> MAAQLALNSEASLWGPYREIWQTVLSALIKRQPEAVHSLDIVLKKYKPDFISLFKNPPKSAQQHERVQKASTEGIPIKGTQRTRILEEQLIKEAFILSDLYNIGEIAAVELLLIGEQQQPTFHGLTRGLVAILLYWDGKSCMAESLLHLIQARKGKTFTLDHSPEVVSMVTRFTDDLMEQGLTNKILTLISQIDVNNEFDKLKKERGLGNKKHRKEVSDLIKECQQSLAHSLYSWSCQTPLNREDTLLLIGYLEKVTVEGDGSLDKVNLTLLMSLLYCLDVGFLEQGTDDREELMKQASMFMDRQYIAAIHNRLQNTQPWKSPGMQATVRLAWALALRGISQFSEVLEFSEADEPMAEIAIGGNVFLFLTEAVVGSESFCTDEFFIRRIHKLVTDFPTLMPMKVKQLRNRAEEDARLIQMSMQMGNEPPASLRRDLEHLLLLIGELYRKDPFHLELALEYWCPTEPLQSTSLMGSFLGVAHQRPPQRQVLLSKFVRQMSDLLPATLYLPYLKMLRGLASGPQCAHYCFSLLKANGGSSAENLQAAGGSPVSWDHFFHSLMLYHEHLRRDLPNTDNIHQRHPPLRGITQRELDGLIACLQLTCTIIDWSESARLALCEHAQWMPVVVILGLLQCSIPPLLKAELLKTLAAFGKSPEIAASLWQSLEYTQILQTVRATGLRQGVGIEVELNEIESRCEEYPLTRAFCQLISTLVESSFPTNLGAGLRAPGFEPYLQFLRDTVFLRYRTRAYRRAAEKWEVAEAVLDVFYKLLKDYEPQPEDFVDQYVELQGEERVAFKPPGFSLMHHLLNESPMLELCLSLMEEGVTQLDTYAPFPGKKHLEKAVAYCFMLLNLTLQKENRFMDLLRESHLSMIVTPLEQLLQGINPRSKKADNVVNIARYLCHGNSNAELAFESAKILCSISCNSKIQEKIVGDFTQDQNVSQKLMVGFVSCLDSEEAEELLDSEKEAEDQVKQTNIRYMTKIHILNLLITSLEMKAPNLAMFLLGYELKKPVSTTNLQDSGVLGCPRTCLHSILDILRKGTDVRAGPVAVWDTPHLAELCYQVIYQLCACADTSGPTMRYLRTSQDFLFSQLQHLPFSVEESEISAMNQMSWLMKTATIELRITSLNRQRSHTQRLLHLLLDDMPTRPYSADGEGGMEDESRSLSGFLHFDTTSKVRRKILRILDSIQFSNEIPEPLQLDFFDRSQIEQVIANCEHKNRRGQTVCNVKLLHRVLVAEVNALQGMAAIGQRPLLMEEINTILQYVVERNKLLQCLHAKRHALESWRQLVEIILTACPQDLIPTEHRQLIIRDLLQDLHVKILDDDAAQELMPIVAGAVFTLTAHLSQSVRTELKQPMTASGLGQSQYVQMLDGSFAAPPGTENISAGFASIGDSSLHMILRNLLEFILKTGGGFQRVRAHLYGSLLYYLQIAQRPDEPDTLESAHKSMWERLTAPEDVFSKLQRDNLSIFESYGTALMEVVCRDACDGHDIGRMLALALLDRIVSVDRQQQWLLYLSNSGYLKVLVDSLAEDDVVLRNLLTPQPPLLKALYIYESKMAFLTRVAKSSQGAIELLRSGVIVRLAQCQVYDMRPETDPHGVFGMRETPVFIPAPVERYRQILLPALQICQLILTSSTAQHLQAAGQVLQFLVAHSDTIQAILRSQEGSLGSLQELALLTGIISKAALPGVLNELDIGLNDGSMMELQGHIGRFQRQCLALLNRFGGSDRLRQLSLQDDSSRLDGVSKKDDMELAMQQICSNVMEYCQALMIQNSPSFQQTVCLFTPSLKESASRDGTRQDSQVSILPSWRLPSLGVVIHLLKQSANNFFTYYDIHRQSVGKLQNVEQLPPDEIKELCQSEMPVGADKISTTQKYGLARRRLVKLINSRAKLLSLCSYIIETCLYILWRHLEYYLLHCTTSDSQDPVFSNMTFGNRRFQDTFNTDPNMDPRNLRQNKVSQQDVDTLLREGANSFGESLQKRLLDIESLYCKVRSRHSFIQALVRRIRGLLRVSRV;>MEELDVDPAETPIPGLGQQNRHIGFSWGPGDLLLYETLYQKQGNSETAARCPFMYLVRSDEDIYSPVLRKLFNESHSIFVGLQKSAEEASGKSRKAQLVQVSRNYRSVLRACMEEMHTLSESTRETAQKYISQISILSAMELSWNLCEILFIESAPAGPLLILLLEWVRLHVCEVDNIVQDVLRSEKPTEHEKFWDGVTGYVLQGRMNEARQLLAKEASTSASARSMCRVLDDLLKKMPMLHTGGTQTLTEFELKWQHWREECERHLQNGTFSSNVHMEAVCRVLLGDEEVLLEKRDLMTTWYHFLVSRLLFKHPTVKPTELHFYAQSSLDMFLAGDSCPEPLDNILLAAFEFDIHQVIKEFSIVSSNWWFVAHLTDLLDHCQLFQAHNLYFGANMREFLLLDYASGLFSHHSLWQLGVDYFDYCPNLGREYLKLHMERIPLSTEKKALKALRICEQRQMTEQVRSICKTMAMQSLCNRRLGSALSWSIRAKDAAFATLISDRFLKEYCERGNFTDLDLIDNLGSAMLLSDRLTFLGKYREFHRMYSQEQFSEAASLLLSLMTARIAPCSFWLTLLLDALPLLEQKQVIFSAEQTYELMRCLEDRMAAKLESTSPDEIQKQDSSIDNTKVEMLRLALARNLARAIVTEGALQE[2x];>MADKFAAKFVSHKISRTRWRPVSASSLQQPDVFATGSWDNEENKVCVWATSDFGATSLDEEYQGDPKQLCDIKHPGDVMDMQFLDKERIVTGSSTGTVTIFRHHENNQTLSVNQRWEQAHYHVGSNMRAPCTAIVCSSPEIVSVGEDGRINCFRAESRDVLRTIDDADSSTMHGVTFLRTTEILTVNSVGQLKLWDLRKQGNDPTQIFSVTGERVPLHCVDRHPNQQHVVATGGQDGMLCIWDVRHGKMPMSLLNAHEAEMWEVHFHPSNPDHLFTCSEDGSLWHWDASADSEKPTFLLGGRSTFNISRSSIAPPNANQSLACAWLSTDPTKGQLEITNLLPSSTLSVNSLDVLGQNLVCGTDAEAIYVTRRLFS[2x];>[2x]MFVARSIAADHKDLIHDVSFDFHGRRMATCSSDQSVKVWDKSENVNWHCTASWKTHSGSVWRVTWAHPEFGQVLASCSFDRTAAVWEEIVGESNDKLRGQSHWVKRTTLVDSRTSVTDVKFAPKHMGLMLATCSADGVVRIYEAPDVMNLSQWSLQHEISCKLSCSCISWNPSSSRAHSPMIAVGSDDSSPNIMGKVQIYEYNENTRKYAKAETLMSVSDPVHDIAFAPNLGRSFHILAVATKDVRIFTMKPLRKELSSSGGVTKFENHTVAQFDNHNSQVWRVSWNITGTVLASSGDDGTVRLWKANYMDNWKCIGVLKGDGNPVGNSFQGIFGSSIGSASHGLQNSVNGTSTSGRKHS;>MAAAERHMTPFQAIDWAGSITLPMVQRVGGFTRAIMAASVNLERSYMELIGAERETSRRNFRDLSLRPDVNLVIGGPKYADCAGGYCYSESSSLLSATRNRFLHWTSYADTLELVEISLDINLVNNAVRLRILNCSILPGGVHICETPNNIVVLILTNQTVHRLILPHPSRMYRSEIISDSHIQSIFTDIGKTNFHDPSNTYVIPAIPGRAPNTTASTAWLSSDGEALFALPSISGGILVIKMPPHDMEGLVTIAELKQSSVMQRLLTGWMPSSIRGDQGPAHLPVSLAVHTLDHDSYLFALCQDHKLRMWSYKDQMCLMVADMLEYVPVSKDIRQTAGTGHKLRLAFSETLGILYLGVYLHTPKQGQFCVFQLMCAESNRYSLDHISSIFTNQETLIDFTFTLTSMDIWALWLDDDNQTVVKHINFEENQAGQWNPVFVNPLPEDDLAISDEQEPQEAYLECLFAPGRFTIAAVQKAIQILRKGSGRVLDLSWEELRKDVTLTVENEIQNAVIDYDVSQEEFRQINIENWCKFYTCCLQYQETLSRPLALLVHPDTNMVCLLRKGFLSFLAPCSLVEHLYLVPAEHLLTVDESVISDDIDAASDIVNLIQCLRMIADYISEDMAYLMESACCHLQSPERVAEQILEDLIANDIDNIMENIQNKLQDTRNPIRAIGFLLQNMDYETNADMEQPQPNTRLNLSTLYGSITASSVVCQAICKISATRFLICRDLLILQHLLLRLGDMALIGAGQLLHSQQELIPRAAQLLLSYYMIRWGSQCLACAVPVDILESNLQHLSVLELSDSQVEKRRYTSGIQTIVELFFEDVARKHFPHVFIQSGASQLQEPLNWSDLIKRITNYLLQLLWPSNPNFQFAECLMRNCQYTQLQEYVRLLLPWCQVNVGSCHFMLAQCYLVAGEGHKALDCFSQAASEVEREDFLEKLIRVEEGESVSPRLQYYNRVLRLLEDVGLPELVIQLATIAIGEASDDWRSQAALRTRIFKHHLDMGHNNQAYDALTQIPDPSRQLDCLRQLVVVLCERSQLQDLVEFPYVNLHNEVVGIIESRARAVDLMTHNYYELLYAFHIYRHNYRKAGSVMFEYGMRLGREVRTLRGLQKQVNSYLACLNCLRLIRPEYAWIVQPVSGAVYERPGASPKRNYDGESSAVPSSSQIEILELRDLEKEYVLAQTRLTLAKHNPSTAAIAGSSAAEEMVALLVQAGLFDTAISLCQTFKLALTSVFEGLACKCIRLQQGGEAAQAEAWEWLAANQLATVITTKESSATDEAWRLMISYLDKYEAKNTLYHHCIINKLLSHGVPLPNWLINRYKAMDAAELLRLYLKYDLLEEAAELVLEYVDALLGKGHQYFGIQAPLSATSQLVWFPYSAIDHLRQALGENESNQHNQAILSKLQRKMDEYFQKLKKATDDYKKLVQKPLRA[2x];>[2x]MKQDSASNATYTVDCEDYVHVVEFNPFDSGEAGSLLAYGGISYVVIASCRFQEEDSTVEGIEFKTLKTFHHGERVVAIAWSPETRCDALLPLLRFATAAGDKKIRIFTSDFQDKNEYKVIEGHSGYINDLVFCSPEGTDIASVGDDHTCRIWDLDGKQIAMFILRSPGMSVAWHPEGAFKLMVAEKTGTIRFYDLTTHQAILSLESVQVPLMSADWCVRNTLRIGAVAGNDWIIWEMPRSSYPQDNKPAHADRARMFRWSKCNENVFATTGYPGKMKSQIAIHHLAHPQPILIGTAPVGSGLSWHRRLPLCVVGGYRKLFFWLTEM;>[2x]SKYGLQDSDEEDDQLNNAEAKKLKAAPVPPQGKPPPLQQATLPGKVTPPPQSPAVDQLDRVLELDSDMADITQDQDLDSVAEEQDITEEQEPLSASSHIASSLGINPHALQVMKASLLLEEEDGEMINRFSSFPSSMDPYPDVRSPRLFPSSHAKRTSSMGLLQSKFASPSISRISETAQGSHSPRILPVTPWSVPAPLAPTFVIPRPAPETHLRTVGTRRQQELVPLEKSVTHGRGSLLIDMGLFMGRSFRVGWGPNWTLVHNGDKLTERLNAEEDQNMDTIDYGFLPKPTSAKSLTESPFKVHMEKLSLEQKSRELQSYLMPLEIELKNSSVDRSAQCPHFKPNAGVAAIHDYAGWVRNLSNEAGELEAVVKQWGLTWTLCESLWGQLKELEASLDEPNEYVRNLERRKAFSHWLAHTAEERIEEEVSLYGPERHVEAVFSFLTGGRISDACRLAQKSGDHRLSLLLSQMVGSQEMRELISLQLVDWNKLQVDHYIQEERLRVFCLLSGTPVWRSSDNRSINVCSQLDWKRTLAVHLWYMLPPTATIAQALRLYERAFQEHEEGEPYACYPLPPYLEDCSISLGDEPSAKFSSLQRDVCVHLLKLYSERQYDLCQLLDPSSVTPDPLDYRLSWHLWMVLQALNYTHLSEHRQGTLHASYAAQLENVGLWEWAIFVLLHIPHPHIREAGVRELLNRQCVVRESPESLAKENFLIHRLCVPAQWVHEAKAIRSRRDGDRHKEALYLLKGHQWNPCHKLVTRHLAADAVINENYRYLQSFLGELSNPEHCKHIQDWETAGKVYLDYIRVIDMLNLIQQDESSGCELEKLHTKVMSLCKWVELIHCYTAKDRLAQSEMAKRVANILRVVLSLQQPPESMSDSSEPRVPLRLLAPHIGRLPMPEDYALEELRGLTQSYLRELICDS;>[2x]MVSVINTVDTSHEDMIHDAQMDYYGIRLATCSSDRSVKIFDVKNGGQILIADLRGHDGPVWQVAWAHPMYGNILASCSYDRKVIIWKEENGTWEKTYEYTGHDSSVNSVCWAPHDFGLVLACGSSDGAISILTFTGDGPWEVKKISNAHTIGCNAVSWAPSVIPGSLVDQPSSQKPNYIKRFVSGGCDNLVKIWREEDGQWKEDQKLEAHSDWVRDVAWAPSIGLPTSTIASCSQDGRVYIWTSDDAATNCWTPKLLHKFNDVVWHVSWSITANILAVSGGDNKVTLWKESVDGQWACISDVNKGQGAVSTVTEGQLNDQ;>MDMLSPVVREAEVSRAARRQSSNRKNPADESWSNATPTRGPSSRTTGQTLFRQHMTPQTWNSSRPPDVSAILGTVGRSPRLLQTPGRLANLSMMSNPDDSVWTTTFSPGRTGMYTTLDSPSFTEDITLSAVMLQEEDPGEAATMSMYPDFLKSFLEHPSSAVFELIEQYEATCNTQITLLKKIVKRVTPGQQKFSKTASILWLLQQEMVTWRLIAALYRDRIQSALEEENMFEIAAPNASEKTIVDKLFQRDTLVRQSQLVVDWLESIAKDEVGDFSDNIEYYAKSVYWENTLHTLKQRSMLSLGSSRPLVSELDPDAPIRQKLPLDDLDREDDIRLLKYLFTLIRAGMTDEAQRLCKRCGQAWRAATLEGWKLYHDANINGGTELQAVEGNPYRCVWKTCCWRMAEDEQFNKYERAIYATLSGNLKQLLPVCESWEDTVWAHFKVMVDSLVEQEIRASIISFNEANELPREYLEANWTLDSVFEELQATDKKRVLEENREHYHIIQKFVILADVDGLMDEFSEWLSNGKNLLLGHLLRFMTHLLLFFRTLGLQAKEEVSVEVLKTYIQRLINEKQIELIAFYVSHLPQELAISQYAVFLENITDPDQRQRCLELAKEAGLDVASITKTVVENTRKKDAGEFAHHDFAPALDSGTSEEDRAKIDVIDWLVFDPAQRAEALKQSNAIMRKFLASKKHEAAKEVFAKIPQDSIAEIYSQWEEQAMDSALPAEDDNAIREHLCIRAYLESHEAFNEWFKHINSPPQKPTLVGQASFTEKVAHEHKEKKYEMDFGIWKGHLDALTSDVKEKIYNVLLFVDGGWMVDVREDTEEDPERSHQMVLLRRLCLPMMCFLLHTVLHNTKQYKDCLRLADIVSSENQKLYTVFSKTEMRNLLQKLRESSLMLLDLQLDPLGYEIQS[3x];>MFPSPRAQGMGSARRPFNSRLTGGRKALGPGVTASSSPSALYSPVGRRVSASGARSTPSRVYLHPAASETVNYNVQLFGSSLPVKVMEALSNASADEPMAACIHEGGWAWLACNDRLIIWKISHSSSAKLMVCKELPLPLSDSEWSADLVDICAQTGDPAAAQSVALMAATPEGSSRYWPNILHEGTYIESYTEFGSSLCAFVTAVKGNSFILSSEKNQLVRLTPDASGKMNQRVLPQGQGMLSGIGRRVSTLFGILSPAVESTLCSVLWDKGDCFYTLTDSSINKWDLDDTSESQVLNWDMSRVLREYISDAIWGSESDYDDIKAGININYLSLNQNCDGLVILSAAWHPGDNPCQIYYTLVTVKDEGYNISDEITVEVTQFNPVFQARGMQLCQLVVPNFSSQACYLYTQEMIFACSTGTGRSTLPQEKIPFEAQGDNIVGAGSCEGWPVFFIRKSGMLTVVARETASVLPEHMEESLSSVSKSSRQAVVKDSRPDQIAHDDKTKHLKAAFLRYCRKDILGAQSMVDSLFSDSDMEPDDELDLAVNQISVDLIDDYPASDPRWAESVPEEAAGFSNTSLILLHQLEDKMKAHSFFVDFLHQVGLFSRLSTCQTKGMLVATRLLLSEHAEKLSAAIVLKNHHAKLPVLVNSAIQLALDKRMCTVPQNLTAADVYFREVSQMEIIFECLVDKEEADLESTSIDSVEWANIVVNVNTILKDMLHVACQYRQSKNSLYKNESGIQEPEHVPWTASSGTAGIRSVVTRQHGIILKVYPQADSGLRTILIEQLAALLNYLLDDYVTQLKSIDKLANEERYNILEMEYAQKRSELLSPLLILGQYAWASNLAEKYCDFDILVQICEMTDNQSRLQRYMTLFAEQNFSDFLFRWYLEKGKRGKLLSQPASQHGQLAAFLQAHDHLSWLHELNSQEFEKAHRTLQTLANMETRYFCKKKTLLGLSKLAALASDFQEDVLQEKVEEIAEQEHFLLHQETLPKKLLEEKQLDLNAMPVLAPFQLIQLYVCEENKRANENDFMKALDLLEYIGDDSEVDVEELKLEILCKAIKRDEWSATDGKDDPIEATKDSIFVKVLQNLLNKGIELKGYLPKAETLLQSEELNSLKTNSYFEFSLKANYECYMKMQS[4x];> MPSATPGAPAASAAMQEALEGAGRIIDRLLQEDRAYPDLSELLNVPVHTCPTISGVSEMDYPLQSPGLLTIPSLPEISAIRRVPLPPELIEQFGHMQCNCMMGVFPEISRAWLTIDSDIFMWNYEDGGDLAYYDGLSETILSVGLVKPKTGIFQPHIRFLLVLSTPVDIVILGLSFANLQPGNLNDSISGGMQLLPDPLYSLPTDNTYLLSITSTDNGRIFLSGKDGCLYEVEYQAEAGWFSQRCRKINHSKSSLSFLVPSVLQFAFSEDDPIVQIAIDNSRNILYTRSEKGVIQVYDLGVDGHGMSRVASVSQNSLVSAAGNIARTIDRNVFKPIIHISVIEMSESVNCHLLAVTHTGVRFYFSTVPFKQPTARPCMLALVHVRLPPGFSASSNVEKPSKVHKALYNNGVLLMAASENEDNDMLWCINRDSFPFQKPMMETQVTTQVDGHSWALSAVDEQKADKIVTPLNKDLIPLTDSPVIIQQHMIPPKRFVLLSAQGSHIFYKLRPVDQLRHLLVSNSGGDGEEIERFFKLHQENQACATCLILACSSAASDREVSSWAARAFFRYGGEAQLRVQSALHAPSNVGPIFGSPLPVASPIPVGSPMPNPSFLGTPTQGACPPNVSTPAYGVATPAPQPPAVPGMMGTEIVFSGKHNGICIYFCRIIGNIWDGSVAVENTFQSGNREVTAIDSSVTPQHLESVLKELKGLLEFLDR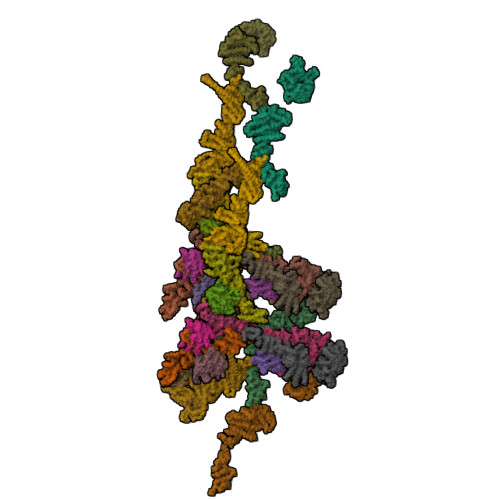YSQFTAGSLGNPGFGTPANRQQRLVSLGRPDIGSSQQAQQELQRKYHTEAQLAEQFSLQGIHQLVRKMCQALALWKLLCEHQFSLVVSDLQKELQEQLKITTFKDLVIRDKELTGALTASLISCYIRDNASVDGISYRLQEVCPLLYSTDDAVCSKANELLQRSRHVPNKQEKERMLRESLKEYQKISQQVDLPNVCAQYRQVRFYEGVVELCLSAAEKKDPQGLGLHFHKNGEPEEDMAGLQAFQERLNSYKCITDTLQELVNQSKAAPQSPSVPKKPGPPVLSSDPNMLSNEEAGIHFEQMLKLAQRSADELFNIALFNWLIQADLTDKLLELNSPFLEPHLVRMAKLDQNKVRYMDLLWRYYEKNRNFSNAARVVAKLADMHSPEISLKQRLEYISRAILSAKSSTTMSTLAADGEFLHELEEKLEVARIQLQIQETLTRQYSHHSTVGDAVSQLDSQLMDITKMFGQYADPFRLSECKLAIIHCAGHSDPILVQTLWQDIIDKELSDSMGNSSVDRMQSLHLKITSLGKIYASTPRYFPLEFLVKYLEQQVCNFSWDAGFVTYTMQEINVPVPKLLEVYDHLFKARDPWWSRMKKPLHLLESIYILLSGYVQEPSKVPSYERRRFTTLCLDAISCYLVELQSMDPAPALLNTVSNFKSLQAKLERLS;>MDGEGFGELLQQAEQLAAETEGVTELPHVERNLQEIQQAGERLRSKTMTRTSQESANVKASVLLGSRGLDISHISQRLESLSAATTFEPLEPVKDTDIQGFLKNEKDNALLSAIEESRKRTFVMAEEYHRESMLVEWEQVKQRVLHTLLASGEDALDFTQESETSYISESGAPGRSSLDNVEMAYARQMYMYNEKVVSGHLQPSLVDLCTEAAERLDDKNVSDLWVMVKQMTDVPLIPASDTLKSRCSGQMQMAFVRQALNYLEQSYKNYTLISVFANLQQAQLGGVPGTYNLVRSFLNIRLPTPIPGLQDGEIEGYPVWALIYYCMRCGDLMAAQQVVNRAQHQLGDFKNCFQEYIHNKDRRLSPTTENKLRLHYRRAVRASTDPYKRAVYCIIGRCDVSDNHSEVADKTEDYLWLKLSQVCFEDEANSSPQDRLTLPQFQKQLFEDYGESHFAVNQQPYLYFQVLFLTAQFEAAIAFLFRLERTRCHAVHVALALFELKLLLKSTGQSAQLLSQEPGEPQGVRRLNFIRLLMLYTRKFEPTDPREALQYFYFLRNEKDNQGESMFLRCVSELVIESREFDMLLGKLEKDGSRKPGAIDKFTRDTKTIINKVASVAENKGLFEEAAKLYDLAKNPDKVLELTNKLLSPVVSQISAPQSNRERLKNMALAIAERYKSQGVSAEKSINSTFYLLLDLITFFDEYHAGHIDLSFDVIERLKLVPLSQDSVEERVAAFRNFSDEIRHNLSEILLATMNILFTQYKRLKGSGPTTLGRPQRVQEDKDSVLRSQARALITFAGMIPYRMSGDTNARLVQMEVLMN[2x];>MQNLEAQVTGSLVAFPDVTQKALKEDEINLDSVLRGKFSTGRTSLAWLACGPQLEITNSVTGERISAYHFSGLTERPPVVVAVKEFTWQKKTGLLVGLVEAEGSVLCLYDIGISKVVKAVVLPGSVTAVEPIINHGGASASTQHLHQSLRWFFGVTAVVTDVGHVLLIDLCLDEVSSNQDELDASDLEVMSVIPTKIPKLREAATRERRHLCLQLAAPTGTTVSCLSYISRTNQLAVGYSDGYFSLWNMKTLRRDYHVQIEGGRVPVCAVAFQEPENDPRNCCYLWAVQSSESGGDVSLHLLQLAFSDRKCLASGQIMYELLEYCEERYSLDLSGSTLSLRGQSNNTKLLGCQTIEKFRVHGEREDGVHEVTSPDTSVSVFSWQVNTYGQGKPSVYLGVFDINRWYQAQMPDSLRSGQFLRNCSYFAFWSLEAVVNITTQDIIFDILVHERSLSRGIPPSYPPPEQFYYPSTYNFDATCLLNSGLIHFACTGFQKETLHFLKKSGSSLNEAIPDGYNRCLAAGLLAPKFTDVQASSLSQEEQLQAILAAAVETSSLGLLTSCIKRWTAEEQPRSAANLRFVLEWTWKKVTLTKQEFDRLCFRLFDGSCNFIDPHTLQSLQQCHLYFSNLTAVLNCFIAQAKEVTQQGAVDLTNKQSVTRLLTLYASVVLWFCRSGMLPDSSDETVQLTRPFYNYQVIQQYYSDQRKKLERLARGKWDTSSLMIDGLINQFGDRIQQLWSRDDNGTGKYPPANLHALLDVYLLENADEMSKHAITIYFLLDIMYSFPDKPDSSIESFPTAFFVPGSLIKLIQGFWLLDHNDYQNSVDCILNPASSRVMSWQHSQIIENLLCHGDSRQALRYLQVMKPVATTSKEVKLHMTVLLANRSILEAWNLQRLHSSRLNVEELLKHMYEMCQEMGLIEELLKLTFTDFEQGYLHKFLQTTGVQNQELLLVHHLQRANYISALQLNQSLKTNHLNDCDRRLRERSGARNAILDQYGKILPRVQRTLASERAKPYSLPSLVWREVARPKPLSTTAKQAAPGSIITKANFICNVLSKIKEVSTANEKREEYSPYQSMVSEEPTAPPLQDIDVPDAFFGTPINKSRRVSRLLDSVVHPVLMEPTPLTSSDTDNNQTPHKSPLLKTSSPLHSSLRRIAHMRSFAKASEFSLLETPLVVRKAKALAANTASSGYTSITPQSILRSSVRTTPLVSPSVSPGRSLTPPLRPKETKISFMELSFTRHAKAAHSSEGNLLAISPVLRSSPDAVWSVKGKVASFTQNTPVKKLDEIDASSSGIQEESQDEMEVSKEISNISVRSEQASLEYHDAPTPEDLENDEISGTTNSQPQVNEVHHQMEDGQLTEKPAELALTEMQEEFIDSEEREIEYISAPLNGPNALECMTAVPDIYLEDASQCILETPEGSSVSVTGEQECVSSAKDSESVISIHDSDDAHSNLSENDQDSEEIEENNLRVPTTVTRCEEFDLIETKDLEVELEEADSEKTNYKDIYPDATVQLGFTVESIEQRYTCELADRRETPSETDEIEGEHFETENNFSLVLEGDVTEEEILEPSSSKTDLELTRPPIAHQKLISENRENIENCETTEKIPANMSPLVDSDHESKTLETLPSEADLSVAEKVLKGTEEKDVPPEVHSEVVLESKLVGNAMMSLDSSESQEVIISQYDNVISIEKLEMTQEKMYGEKTEQINEGQVSPNRDQSTLVKPLTPRRSIRKSSKPADSSTDIIGNITLPTTPKRGLKKAKENVDTLKNSISVVPEEELTLGTRRITRKATLTALDNPEPLQIKEPPSGEDLQVQPSTPTRGRRGKVITSDDLKEPPSGEDLQVQPSTPTRGRRGRVITSDDLREPPPGEDLQVQPSTPTRGRRGRVITSDDIKESPSVEDLQVQPSTPTRGRRGKVITSDDIKEPPSVEDLQVQPSTPTRGRKGKVITSDDIKEPLSGEDLQVQPSTPTRGRKGKVITSDDIKEPLSEEVLQEQPSTPTRGRRGRVITSDGKGYECVEEKNALPLTPTRITRSKNILEPEKGISQIEPEKGISQIEPDKGLSQIEDTGETEHEVVTPRRGRRGKRVVNELVKHFERNSSQPNIKADTSPPVSPKKVSLRWTRTRSENQRINATEEQASKIQEDLSDTPRKRYKKSSNKMGFEETTDTVTEGAIVEDVQESLIISHLGKNPNTSIVRSARKTALPPVTEDHSEQPLLPPESHSKVHSSLAIADEENKTNTRTRSGNKSSVDVSAITFEFSTPKARTKKTAKGSAVPTELIPSTQYVFSPPSTRTRRATRANVSEAVIEPQLQFQESCEIAETEVPEVPASKPRGRPPKHKAKAVTRVLKKPSWSTPPVEIKLISPPESPAVSETNTKTDSTEAKGAEKISVRRTRRRIIAKPVTRRKMR[2x]> MKKQRNLRSMAAQAVEQVVEQGQSLSNILPPLQQKVSDKDKALLQELCFGVLRTLSQLDWLINKLMARPMTGKQRTVHYLIMVGLYQLLYTRIPPHAALAETVEGAIAIKRPQLKGLINGVLRQFQRQQEELLAEFNASDARYLHPSWLLKRLQKAYPEQWQSIVEANNQRPPMWLRINRTHHSRDSWLALLDEAGMKGFPHADYPDAVRLETPAPVHALPGFEDGWVTVQDASAQGCMTWLAPQNGEHILDLCAAPGGKTTHILEVAPEAQVVAVDIDEQRLSRVYDNLKRLGMKATVKQGDGRYPSQWCGEQQFDRILLDAPCSATGVIRRHPDIKWLRRDRDIPELAQLQSEILDAIWPHLKTGGTLVYATCSVLPEENSLQIKAFLQRTADAELCET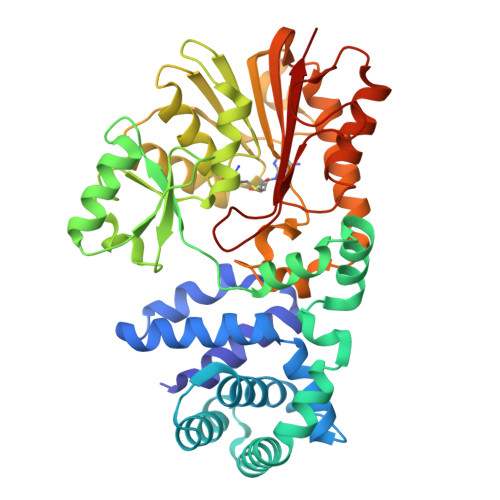GTPEQPGKQNLPGAEEGDGFFYAKLIKK>[2x]GQSGKSLSVKKVMCTASPEGEAVPSLLDGNGIEFQPLDVVNWKDYPYKPEVSFRIAHTGREILLHYKVKEASVRAVASGDNGRVWEDACVEFFVSPEGD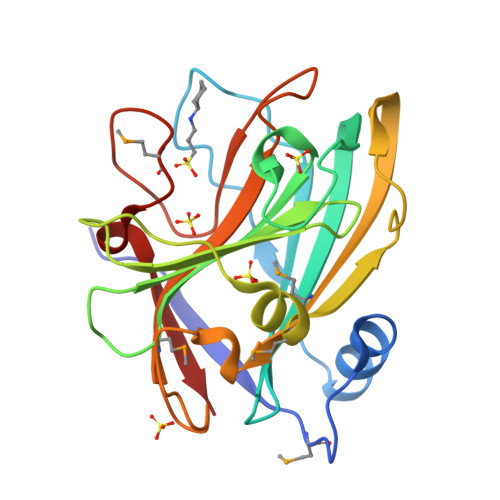DRYYNFECNCAGRLLIQGGAVNERRPTASQEVLGMVKRWSSLAGEPFEERLGECSWELVMVIPVSAFFQHSVGSLDGKTMKGNFYKCGDKLQTPHFLSWSPIGLERPMFHCPAFFGTLSFE>[4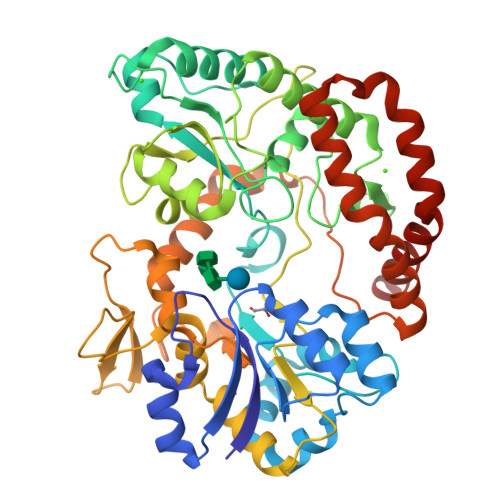x]GPKTLKFMTASSPLSPKDPNEKLILQRLEKETGVHIDWTNYQSDFAEKRNLDISSGDLPDAIHNDGASDVDLMNWAKKGVIIPVEDLIDKYMPNLKKILDEKPEYKALMTAPDGHIYSFPWIEELGDGKESIHSVNDMAWINKDWLKKLGLEMPKTTDDLIKVLEAFKNGDPNGNGEADEIPFSFISGNGNEDFKFLFAAFGIGDNDDHLVVGNDGKVDFTADNDNYKEGVKFIRQLQEKGLIDKEAFEHDWNSYIAKGHDQKFGVYFTWDKNNVTGSNESYDVLPVLAGPSGQKHVARTNGMGFARDKMVITSVNKNLELTAKWIDAQYAPLQSVQNNWGTYGDDKQQNIFELDQASNSLKHLPLNGTAPAELRQKTEVGGPLAILDSYYGKVTTMPDDAKWRLDLIKEYYVPYMSNVNNYPRVFMTQEDLDKIAHIEADMNDYIYRKRAEWIVNGNIDTEWDDYKKELEKYGLSDYLAIKQKYYDQYQANKN> MTDSYATKASNLKKTAILASKEAKRWQLRTNKGTKDLQARAKRVMRDMMGFWKRNEREERDLRKAAERLELENARKEEADREAARQRRKLNFLISQTELYSHFISKKIKTHEVERSTDHPDVATDEKDKIPEPTLNINVPEPTGPIAPKVTDFNSLDFDNEDESALQAAAMANAQNAIAEAQKKAREFNKDETKLDEDGEMNFQHPELTEFEVAQPKLLNCQLKEYQLKGLNWLVNLYEQGINGILADEMGLGKTVQSISVMAYLAERYDIWGPFLVVAPASTLHNWQQEVSKFVPDFKVLPYWGTAADRKVLRKFWDRKHTTYKKDSPFHVMITSYQLVVSDVAYFQKMKWQYMILDEAQAIKSSQSSRWKCLLGFHCRNRLLLTGTPIQNNMQELWALLHFIMPSLFDSHDEFSEWFSKDIESHAQSNTKLNEDQLKRLHMILKPFMLRRVKKHVQKELGDKIEIDVFCELSYRQRAMYQSLRNQISIMDLIEKATVGDNEDSATLMNLVMQFRKVCNHPDLFERADTSSPFFCGHFAETGSFLREGTNVALGYSTRSLVEYRLPRLIWCDGGRLDKPGPGNLVAGFRSKYLNHMMNIWTPENIRSSLEGIENFTWLRFVDTSLQEAYRASHTDVFARAVDLASKQNRLGHMQIVYDEPEDKKWTPVHALFQICERENPKAVAEITTEGVLRDLMNIARVKYRELGLCRLEKAARPRASAPPIEVVCDSRSAVIERENIMFHPAMRKALFGPTPSEIKEASFGPRPVTLYPP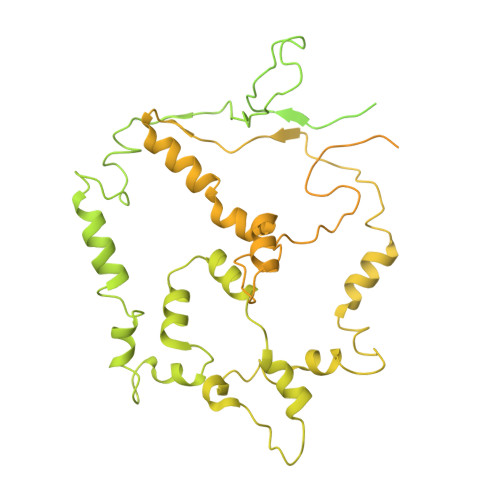RALLPAPDHDKQRFTNITVPSMARFVTDSGKLAKLDELLRELKEGGHRVLLYFQMTRMIDLMEEYLTYRNYKYCRLDGSTKLEDRRDTVADFQTRPEIFIFLLSTRAGGLGINLTTADTVIFYDSDWNPTIDSQAMDRAHRLGQTKQVTVYRLITRGTIEERIRKRALQKEEVQRVVITGTGSVDFSGRRPPENRNRDIAMWLADDEQAEMIERREKELIESGEYDKIMQQRRKGGKRKRGAANGDTVPSLEDMYHEGEGHFDDNKGSGAATPVDADSLGRGGKRKKAGGSKKAKTTKQRLAIADGEIDDGEIDIDYKDDDDKGTDYKDDDDK> MKGTDFVHSVKKFLRVRIFTKIESEDDYILSGESVMDRDSESEEAETKDIRKQIQLLKKIIFEKELMYQIKKECALLISYGVSIENENKVIIELPNEKFEIELLSLDDDSIVNHEQDLPKINDKRANLMLVMLRLLLVVIFKKTLRSRISSPHGLINLNVDDDILIIRPILGKVRFANYKLLLKKIIKDYVLDIVPGSSITETEVEREQPQENKNIDDENITKLNKEIRAFDKLLNIPRRELKINLPLTEHKSPNLSLMLESPNYCNALIHIKFSAGTEANAVSFDTTFSDFKEVED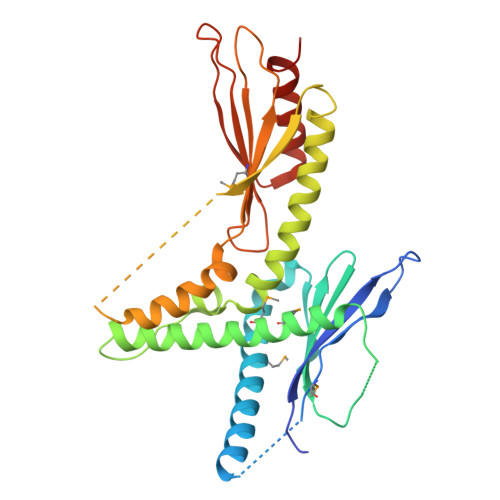FLHFIVAEYIQQKKV>KDDTQSSVTIEFMHSSVEQERQAVITKLIEKFEKENPSITVKQVPVEEDAYNTKVITLARTGALPEVIEVSHDYAKVMDKEQLLDRDAIGEAIKAVGEKTFYDGILRVVRTEDGTAWTGVPISAWLSGVWYHKDVLAAAGIKEPHNWQQLLKASQMLNDPAKKHYGIALPTAESVMTEQAFSQFALSGGANVFDAQGNIQIDTPEMLNALAFYKELAKNTMPGSNDVMEIKDAFMNGSAPMAVYSTYILPAVFKEGDPANLGFVVPTEKSSAVYGMVTSLTITTGQTEEETKAAEKFVTWMEQAQNASDWVMMSPGAALPVNKLVVDTESWKN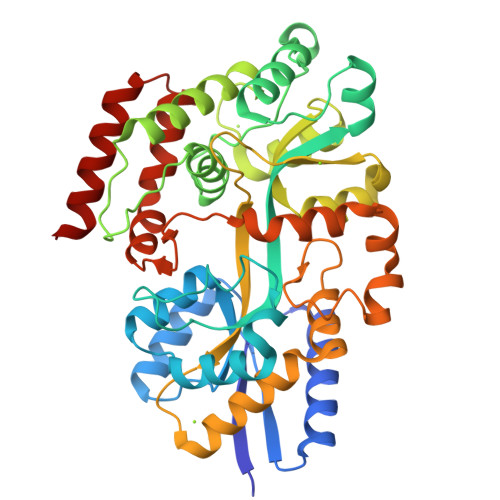NEVIKAFGQLPYELIAQFPNVQVFGAVGDKNFTRMGDVTGSGIISSMVHNVTVGQQDLNTTLSNSQKRLTDLVSQR[2x]2-[4-[3-~{tert}-butyl-5-(2-pyridin-2-ylethyl)phenyl]phenyl]sulfonylethanol | C25 H29 N O3 S | 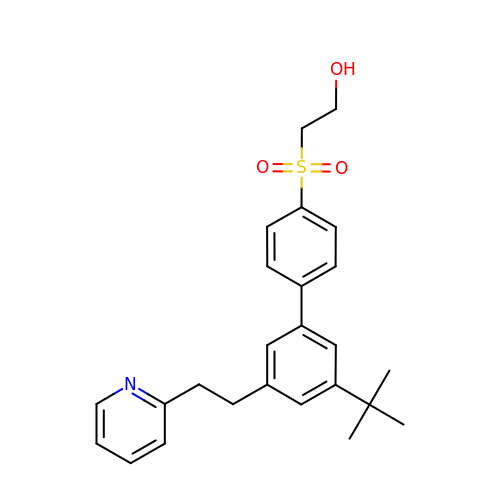MDYWYEIFJBZYTD-UHFFFAOYSA-N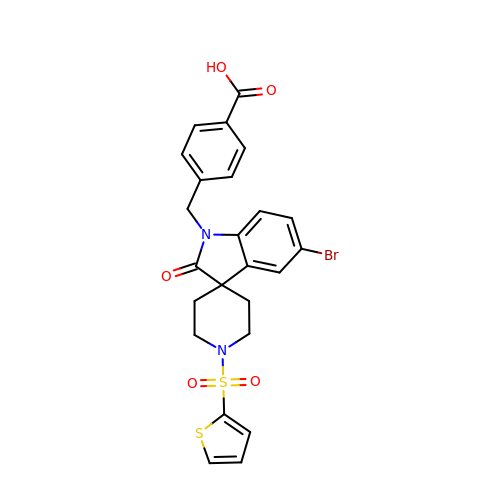4-({5-bromo-2-oxo-1'-[(thiophen-2-yl)sulfonyl]spiro[indole-3,4'-piperidin]-1(2H)-yl}methyl)benzoic acid | C24 H21 Br N2 O5 S2 | GNPZBVGDUWGWDJ-UHFFFAOYSA-N> MKCLVTGGNVKVLGKAVHSLSRIGDELYLEPLEDGLSLRTVNSSRSAYACFLFAPLFFQQYQAATPGQDLLRCKILMKSFLSVFRSLAMLEKTVEKCCISLNGRSSRLVVQLHCKFGVRKTHNLSFQDCESLQAVFDPASCPHMLRAPARVLGEAVLPFSPALAEVTLGIGR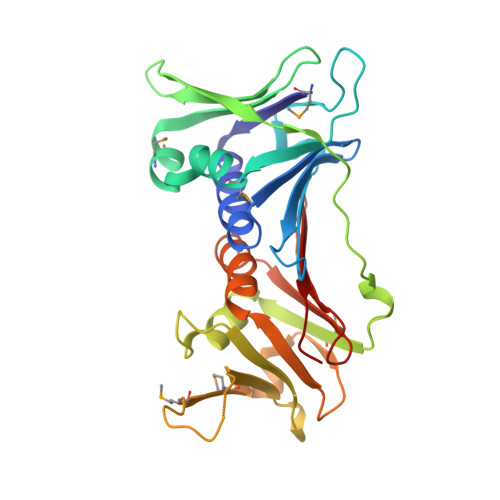GRRVILRSYHEEEADSTAKAMVTEMCLGEEDFQQLQAQEGVAITFCLKEFRGLLSFAESANLNLSIHFDAPGRPAIFTIKDSLLDGHFVLATLS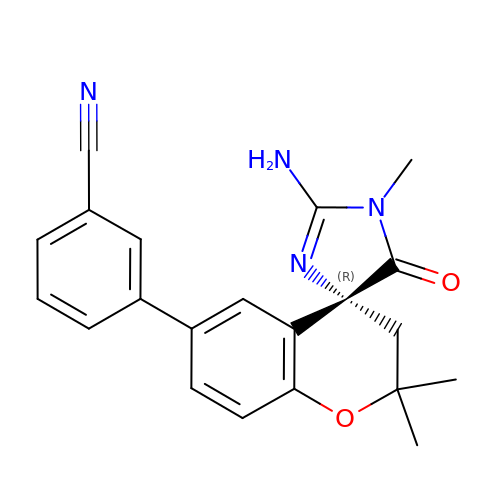3-[(4R)-2'-amino-1',2,2-trimethyl-5'-oxo-1',2,3,5'-tetrahydrospiro[chromene-4,4'-imidazol]-6-yl]benzonitrile | C21 H20 N4 O2 | LASIJFPKQNWUQE-OAQYLSRUSA-N> MMEKSKDFLGTGWGFPPEFETSIGQVKTTSGVEDIQKSLEILFSTKIGERIMQPTYGCNLDELLFSPINR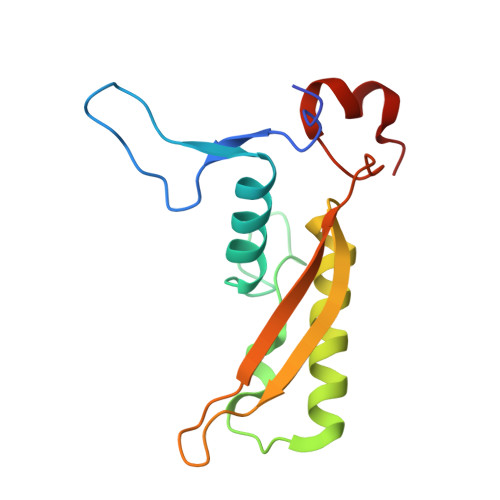TLKTYVIELIKNAILYHEPRIDPEKIDITQGNEIEGELLIHLQYIVRATNSRKNMVYPFYLEEGTNI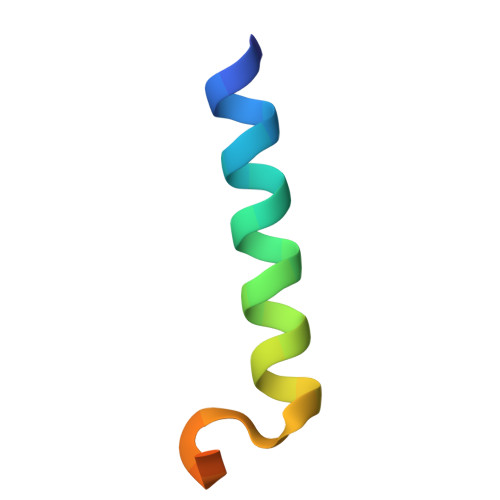> DLSKQMEEEAVRLFIEWLKNGGPSSGAPPPS>[2x]EPKLDMNKQKISPAEVAKHNKPDDCWVVINGYVYDLTRFLPNHPGGQDVIKFNAGKDVTAIFEPLHAPNVIDKYIAPEKKLGPLQGSMPPELVCPPYAPGETKEDIARKEQLKSLLPPLDNIINLYDFEYLASQTLTKQAWAFYSSGANDEVTHRENHNAYHRIFFKPKILVDVRKVDISTDMLGSHVDVPFYVSATALCKLGNPLEGEKDVARGCGQGVTKVPQMIST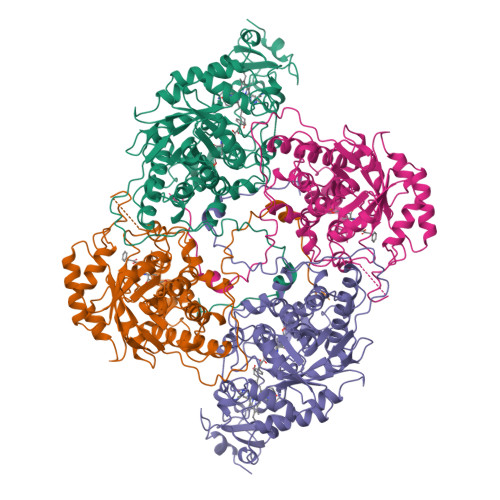LASCSPEEIIEAAPSDKQIQWYQLYVNSDRKITDDLVKNVEKLGVKALFVTVDAPSLGQREKDMKLKFSNTKAGPKAMKKTNVEESQGASRALSKFIDPSLTWKDIEELKKKTKLPIVIKGVQRTEDVIKAAEIGVSGVVLSNHGGRQLDFSRAPIEVLAETMPILEQRNLKDKLEVFVDGGVRRGTDVLKALCLGAKGVGLGRPFLYANSCYGRNGVEKAIEILRDEIEMSMRLLGVTSIAELKPDLLDLSTLKARTVGVPNDVLYNEVYEGPTLTEFEDA> GPGAPNVLNWEQVQRLDGILSETIPIHGRGNFPTLELQPSLIVKVVRRRLAEKRIGVRDVRLNGSAASHVLHQDSGLGYKDLDLIFCADLRGEGEFQTVKDVVLDCLLDFLPEGVNKEKITPLTLKEAYVQKMVKVCNDSDRWSLISLSNNSGKNVELKFVDSLRRQFE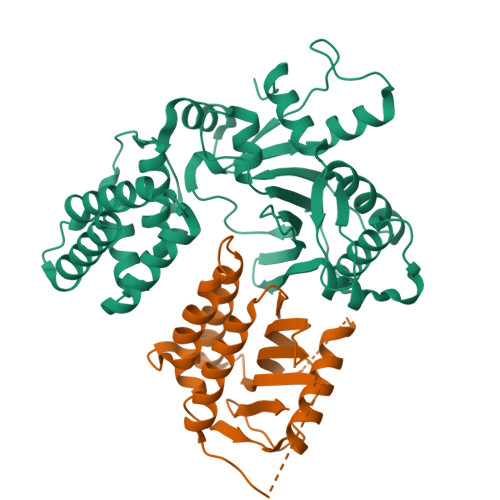FSVDSFQIKLDSLLLFYECSENPMTETFHPTIIGESVYGDFQEAFDHLCNKIIATRNPEEIRGGGLLKYCNLLVRGFRPASDEIKTLQRYMCSRFFIDFSDIGEQQRKLESYLQNHFVGLEDRKYEYLMTLHGVVNESTVCLMGHERRQTLNLITMLAIRVLADQNV;> GPGAPDEVIDEEVNIEFEAYSLSDNDYDGIKKLLQQLFLKAPVNTAELTDLLIQQNHIGSVIKQTDVEVFGFISLLNLTERKGTQCVEQIQELVLRFCEKNCEKSMVEQLDKFLNDTTKPVGLLLSERFINVPPQIALPMYQQLQKELAGAHRTNKPCGKCYFYLLISKTFVEAGQHNGGSRGQVTALVSLKAGLIQSRSTLSDFQGTFMTVGIALS5'-O-{[(2S)-azetidine-2-carbonyl]sulfamoyl}adenosine | C14 H19 N7 O7 S | 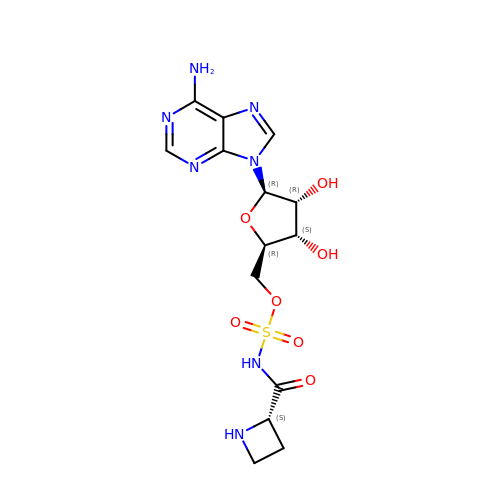DQFRXHHGQUUTOL-XLZJSAHRSA-N>[2x]SMSP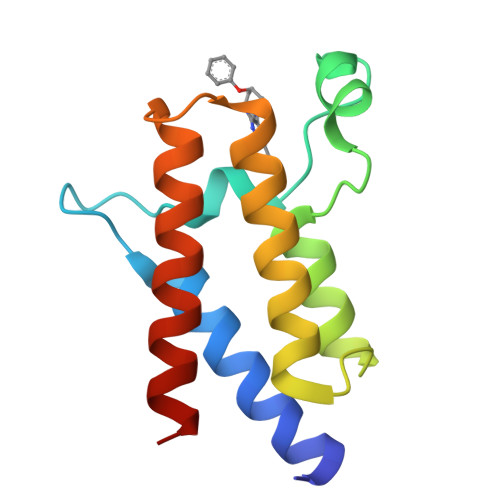AYLKEILEQLLEAIVVATNPSGRLISELFQKLPSKVQYPDYYAIIKEPIDLKTIAQRIQNGSYKSIHAMAKDIDLLAKNAKTYNEPGSQVFKDANSIKKIFYMKKAEIEHHE> MTSQSTGTVLETPRTGPESRCPIDHTAFTSPTGCPVSPRAAAFDPFTGPYQVDPAASLRWSRDEEPVFYSPELGYWVVTRYEDVKAVFRGNELFSPSIALEKITPTSDEANAVLARYGYAMNRTLVNEDEPAHMPRRRALMEPFTPAALAHHEPMVRRLTREYVDRFIDTGHVDLVDEMLWEVPLTVALHFLGVPEEDMDTLREYSIAHTVNTWGRPAPEQQVAVADAVGKFWQFAGTVLDKMRKDPDGHGWMPFGIRVQQEQPDVVTDSYLHSMMMAGIVAAHETTANASANALRLLLEHRDVWEEICADPSLIPNAVEECLRHSGSVAAWRRLVTADTTINGVEVPAGAKLLIVNSSANHDERHFISLDDFDIRRDNASDHLTFGYGSHQCMGKNLARMEIQIFLEELTRRLPHMELVPDQEFTYLPNTSFRGPDHVWVRWDPARNPERADPELLSRRQPVKIGEPSKNTIARTMAVSGLESIADDILLITLRDTSGRPLPKWSAGSHIDVDCGAVSRQYSLCGDPHDRTTFQVAVLHDRESRGGSRWIHTELAVGATLRVRGPRNHFKLDPDAKRYVFVAGGIGITPVIAMADQVKAAGGDYEIHYAGRSRTSMAFLDRLARDHGESVRVYPGDEGVRMDLPSLFADPEDGTQVYSCGPERLLSALSEATAHWPDDTLHVEHFSSTLEELDPSKEHGFDVVLKDSGITVPVAADQTVLQALRAANIDAQSDCEEGICGACEVPVLDGEVDHRDLVLTKTERAAGKTMMTCCSRA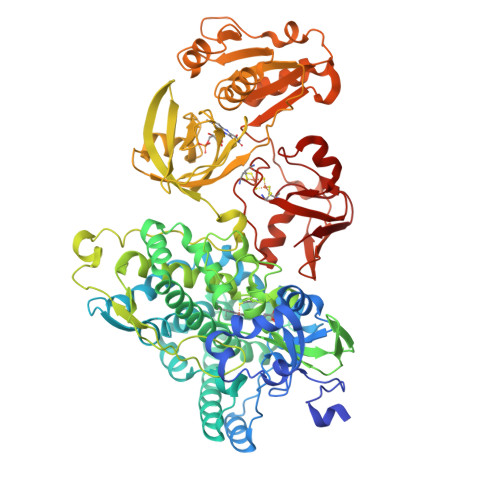CGDKLTLQL>[2x]MSLKIDAVDLFYLSMPEVTDAADGSQDALLVRVAAGGHIGWGECEAAPLPSIAAFVCPKSHGVCRPVSDSVLGQRLDGPDDIARIAALVGYNSMDLLQAPHMLSGIEMALWDLLGRRLSAPAWALLGYSASHGKRPYASLLFGDTPQETLERARAARRDGFAAVKFGWGPIGRGTVA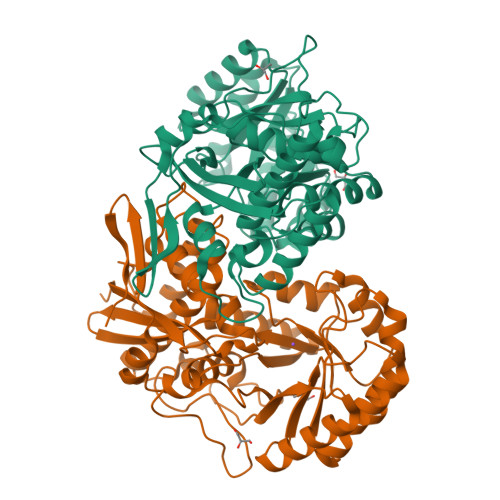ADADQIMAAREGLGPDGDLMVDVGQIFGEDVEAAAARLPTLDAAGVLWLEEPFDAGALAAHAALAGRGARVRIAGGEAAHNFHMAQHLMDYGRIGFIQIDCGRIGGLGPAKRVADAAQARGITYVNHTFTSHLALSASLQPFAGLEADRICEYPAAPQQLALDITGDHIRPDAEGLIRAPEAPGLGLQVAASALRRYLVETEIRIGGQLIYRTPQLEGHHHHHH Here, we report that c-di-GMP can assemble into a tetramer that mediates the effective dimerization of a transcription factor, BldD, which controls the progression of multicellular differentiation in sporulating actinomycete bacteria. BldD is an 18 kDa DNA-binding protein consisting of two distinct domains connected by a flexible linker. BldD sits at the top of the regulatory cascade controlling development, serving to repress expression of sporulation genes during vegetative growth (den Hengst et al., 2010). Specifically, structural and biochemical analyses show that the second messenger c-di-GMP activates BldD DNA binding by driving a unique form of dimerization that is mediated by a tetrameric form of c-di-GMP.

The N-terminal domain is the DNA-binding domain (DBD) and has a xenobiotic response element (XRE) helix-turn-helix (HTH) DNA-binding motif (Kim et al., 2006). Our data and those of others (Lee et al., 2007a) show that the BldD DBD alone can dimerize at higher concentrations (≥10 μM). Consistent with these findings, the crystal structure of the S. coelicolor BldD DBD revealed a dimer with a small contact interface (Kim et al., 2006). We obtained additional views of the BldD DBD by solving the S. venezuelae BldD DBD structure to 2.80 Å resolution. This structure contained two DBD dimers in the asymmetric unit. Comparison of these dimers with the dimer from the S. coelicolor DBD structure showed that, although hydrophobic residues within the C-terminal regions of the DBDs make contacts between the subunits in each case, all three dimers take distinct conformations. Moreover, there is less than 300 Å2 BSA per subunit in this dimer, which is far less than the 1000 Å2 BSA per subunit typically observed for biologically relevant dimers. These data indicate that the BldD DBD is unlikely to form a stable DNA-binding active dimer at physiologically relevant concentrations. The DBD-DBD interacting surfaces observed in the BldD-DNA complex correspond to the hydrophobic regions near the DBD C terminus that interact in the apo DBD structures. However, the interfaces are yet again different, supporting the notion that DBD dimerization is weak and malleable.

>MSSEYAKQLGAKLRAIRTQQGLSLHGVEEKSQGRWKAVVVGSYERGDRAVTVQRLAELADFYGVPVQELLP[3x]> MGSDKIHHHHHHENLYFQGMHPTIARMQ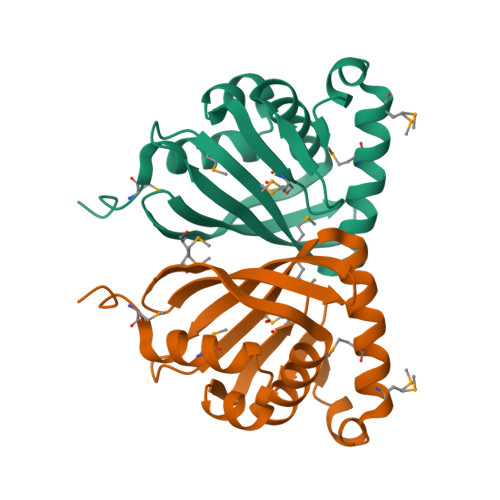EVVAKGDESLIHALLAEDVRFMPPTYYKTWTGRDPVAAVLGHVGQVFSEFRYRRIMGEGKDWALEFQCKVGELDAVGVDLITLNEGGLIQDFEVVMRPYKTVGALRDAMNARVMTDARFLKYREALS> QQKLPTNPFEVLRQPP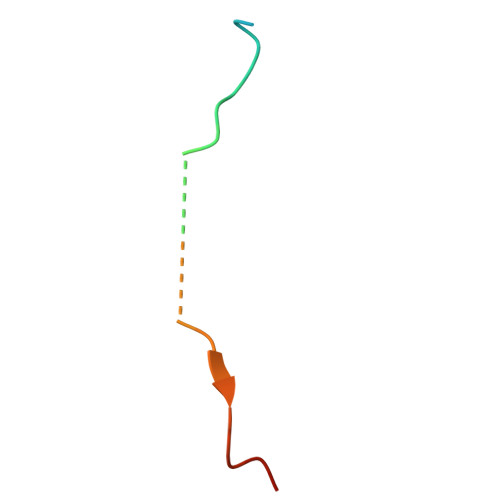KKKKREHACFENPGLNLE Adenylosuccinate synthetase (AdSS) participates in both biosynthesis and salvage pathways of purines. Helicobacter pylori adenylosuccinate synthetase (AdSS) is present in solution in a dynamic equilibrium of monomers and biologically active homodimers. The addition of the His6-tag on the C-terminus (C-His-AdSS) was proven to have a negligible effect on the characteristics of this enzyme. This paper shows that the same enzyme with the His6-tag fused on its N-terminus (N-His-AdSS) has a high tendency to precipitate.

Two monomers of the enzyme occupy the asymmetric unit, forming a catalytically active dimer, with the Arg135 side chain participating in building the active site of the neighboring monomer. N-His-AdSS enzyme was incubated with GTP, IMP, Had (hadacidin, analog of Asp), and MgCl2 during crystallization, just like the C-His-AdSS variant was. However, clearly defined electron density for the Had molecule (HDA in the PDB denotation) is not visible in the structure. The shape of the electron density blob found in the approximate Asp-binding site of N-His-AdSS fits one sulfate ion, which could originate from the crystallization solution containing 0.2 M ammonium sulfate. One additional sulfate ion is found in the active site exactly at the position, which is occupied by the 6-Pi group of 6-P-IMP (IMO in the PDB denotation) in the structure of the C-His-AdSS variant. In accordance with the missing Had molecule, in the N-His-AdSS structure, the Asp-binding loop (residues 289–294) is moved away from the active site (Cα of Thr291 moved by 6.1 Å) and is poorly defined in the electron density. The electron density blob in the supposed Mg-binding site did not fit the Mg ion, so the Ca ion was placed there instead, as it made a much better match. The calcium ion is coordinated with six oxygen atoms: from α- and β-phosphate of GDP, the backbone carbonyl group of Gly39, the side-chain carbonyl group of Asp12, and two sulfate ions present in the active site in the places of Had and 6-Pi group of 6-P-IMP. Since no His6-tag handle is visible in the N-His-AdSS structure, it can be concluded that it is too flexible to be observed, and obviously not so firmly bound to the protein as in the mentioned case of G. stearothermophilus purine nucleoside phosphorylase. The buried surface area between monomers in the structure of N-His-AdSS is 2422 Å2 (as calculated with Pisa, version 1.52), which compares well with 2342 Å2 calculated for the structure of C-His-AdSS.

>[2x]SHMADVVVGIQWGDEGKGKIVDRIAKDYDFVVRYQGGHNAGHTIVHKGVKHSLHLMPSGVLYPKCKNIISSAVVVSVKDLCEEISAFEDLENRLFVSDRAHVILPYHAKKDAFKEKSQNIGTTKKGIGPCYEDKMARSGIRMGDLLDDKILEEKLNAHFKAIEPFKKAYDLGENYEKDLMGYFKTYAPKICPFIKDTTSMLIEANQKGEKILLEGAQGTLLDIDLGTYPFVTSSNTTSASACVSTGLNPKAINEVIGITKAYSTRVGNGPFPSEDTTPMGDHLRTKGAEFGTTTKRPRRCGWLDLVALKYACALNGCTQLALMKLDVLDGIDAIKVCVAYERKGERLEIFPSDLKDCVPIYQTFKGWEKSVGVRKLDDLEPNVREYIRFIEKEVGVKIRLISTSPEREDTIFL>[8x]MREYDIIAIGGGSGGIATMNRAGEHGAQAAVIEEKKLGGTCVNVGCVPKKIMWYGAQIAETFHQFGEDYGFKTTDLNFDFATLRRNRESYI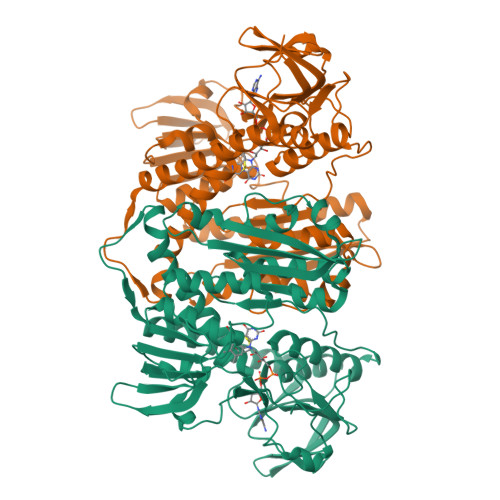DRARSSYDGSFKRNGVDLIEGHAEFVDSHTVSVNGELIRAKHIVIATGAHPSIPNIPGAELGGSSDDVFAWEELPESVAILGAGYIAVELAGVLHTFGVKTDLFVRRDRPLRGFDSYIVEGLVKEMERTNLPLHTHKVPVKLEKTTDGITIHFEDGTSHTASQVIWATGRRPNVKGLQLEKAGVTLNERGFIQVDEYQNTVVEGIYALGDVTGEKELTPVAIKAGRTLSERLFNGKTTAKMDYSTIPTVVFSHPAIGTVGLTEEQAIKEYGQDQIKVYKSSFASMYSACTRNRQESRFKLITAGSEEKVVGLHGIGYGVDEMIQGFAVAIKMGATKADFDATVAIHPTSSEEFVTMR>[2x]MQPKLTIWCSEKQVDILQKLGEEFKAKYGVEVEVQYVNFQDIKSK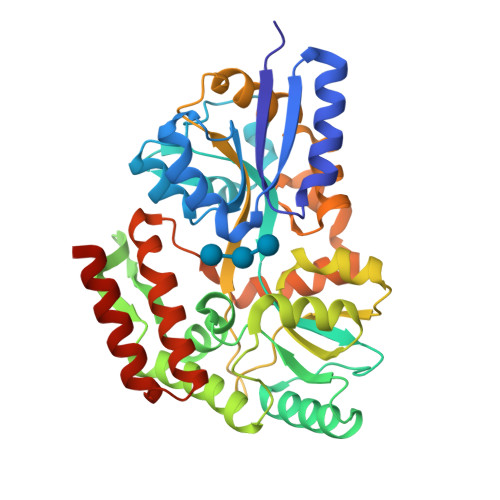FLTAAPEGQGADIIVGAHDWVGELAVNGLIEPIPNFSDLKNFYETALNAFSYGGKLYGIPYAMEAIALIYNKDYVPEPPKTMDELIEIAKQIDEEFGGEVRGFITSAAEFYYIAPFIFGYGGYVFKQTEKGLDVNDIGLANEGAIKGVKLLKRLVDEGILDPSDNYQIMDSMFREGQAAMIINGPWAIKAYKDAGIDYGVAPIPDLEPGVPARPFVGVQGFMVNAKSPNKLLAIEFLTSFIAKKETMYRIYLGDPRLPSRKDVLELVKDNPDVVGFTLSAANGIPMPNVPQMAAVWAAMNDALNLVVNGKATVEEALKNAVERIKAQIQGSHHHHHH>MKRIVVKVGSHVISEENTLSFERLKNLVAFLAKLMEKYE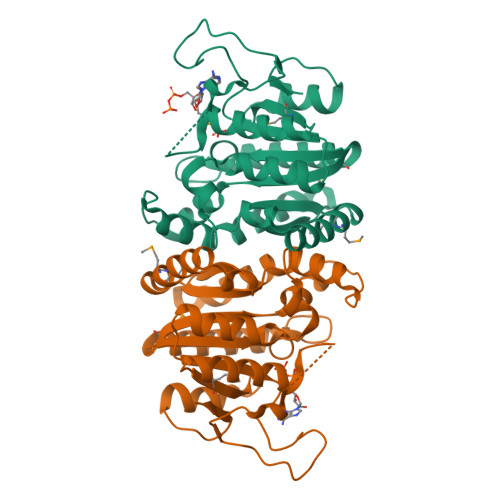VILVTSAAISAGHTKLDIDRKNLINKQVLAAIGQPFLISVYNELLAKFNKLGGQILLTGKDFDSRKATKHAKNAIDMMINLGILPIINENDATAIEEIVFGDNDSLSAYATHFFDADLLVILSDIDGFYDKNPSEFSDAKRLEKITHIKEEWLQATIKTGSEHGTGGIVTKLKAAKFLLEHNKKMFLASGFDLSVAKTFLLEDKQIGGTLFE[4x]3-(3,4-dimethoxyphenyl)-N~5~-(1-methylpiperidin-4-yl)-6-phenylpyrazolo[1,5-a]pyrimidine-5,7-diamine 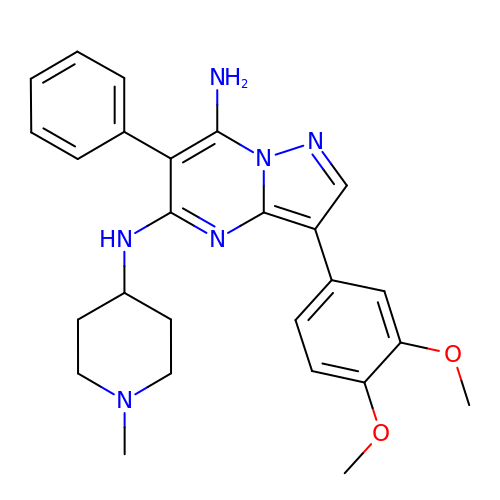| C26 H30 N6 O2 | ZVVQDNWRXSSQDL-UHFFFAOYSA-N>[3x]ASNFTQFVLVDNGGTGDVTVAPSNFANGVAEWISSNSRSQAYKVTCSVRQSSAQNRKYTIKVEVPKVATQTVGGVELNVAAWRSYLNMELTIPIFATNSDCELIVKAMQGLLKDGNPIPSAI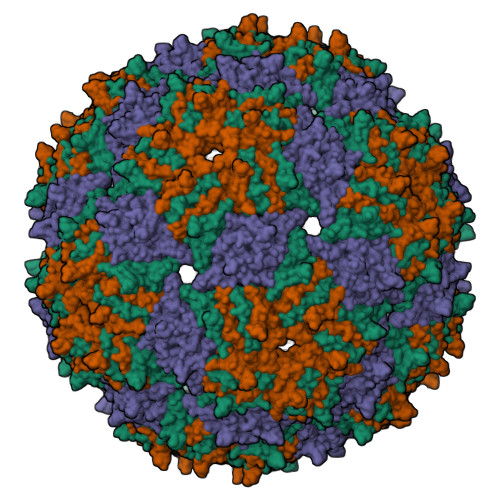AANSGIY CTP synthase (CTPS) is a key enzyme in de novo CTP synthesis, playing a critical role in nucleotide metabolism and cellular proliferation. Human CTPS1 (hCTPS1), one of the two CTPS isoforms, is essential for immune responses and is highly expressed in proliferating cells, making it a promising therapeutic target for immune-related diseases and cancer. hCTPS1 functions as a homotetramer, with each monomer comprising a glutamine amidotransferase (GAT) domain and an amidoligase (AL) domain. In the presence of GTP, the GAT domain hydrolyzes glutamine (Gln) to produce ammonia, which is transferred to the AL domain to catalyze the conversion of uridine triphosphate (UTP) to cytidine triphosphate (CTP) via an ATP-dependent intermediate, 4-phospho-UTP (4-Pi-UTP).

To stabilize the GAT domain, we included 6-diazo-5-oxo-L-norleucine (DON), a glutamine analog that irreversibly inhibits CTPS activity by covalently binding to the glutamine site. Using 312,573 particles for reconstruction, we achieved a final resolution of 3.3 Å. The structure showed that hCTPS1 filaments consist of helical arrays of tetramers, with each helical unit rising by 105 Å and twisting by approximately 40°. The tetramers are connected through α-helix-mediated interactions involving residues 346–357 in the GAT domain. Notably, residues H355 and W358, which are critical for filament assembly across species, exhibited continuous electron density in the density map, underscoring their conserved role. In our structure, two CTP molecules were observed bound to each protomer: one at the interface of three protomers (overlapping with the UTP binding site) and the other within a single protomer (overlapping with the ATP binding site). We designated these as the canonical and non-canonical binding pockets, respectively. In the canonical binding pocket, the triphosphate group of CTP is stabilized by electrostatic and hydrogen-bonding interactions with each protomer. In the non-canonical binding pocket, the triphosphate group interacts electrostatically with a loop, while the cytosine group is stabilized by interactions with S21, K319, and F77.

>MKYILVTGGVISGIGKGIIASSVGTILKSCGLHVTSIKIDPYINIDAGTFSPYEHGEVFVLDDGGEVDLDLGNYERFLDIRLTKDNNLTTGKIYQYVINKERKGDYLGKTVQVVPHITDAIQEWVMRQALIPVDEDGLEPQVCVIELGGTVGDIESMPFIEAFRQFQFKVKRENFCNIHVSLVPQPSSTGEQKTKPTQNSVRELRGLGLSPDLVVCRCSNPLDTSVKEKISMFCHVEPEQVICVHDVSSIYRVPLLLEEQGVVDYFLRRLDLPIERQPRKMLMKWKEMADRYDRLLETCSIALVGKYTKFSDSYASVIKALEHSALAINHKLEIKYIDSADLEPITSQEEPVRYHEAWQKLCSAHGVLVPGGFGVRGTEGKIQAIAWARNQKKPFLGVCLGMQLAVVEFSRNVLGWQDANSTEFDPTTSHPVVVDMPEHNPGQMGGTMRLGKRRTLFQTKNSVMRKLYGDADYLEERHRHRFEVNPVWKKCLEEQGLKFVGQDVEGERMEIVELEDHPFFVGVQYHPEFLSRPIKPSPPYFGLLLASVGRLSHYLQKGCRLSPRDTYSDRSGSSSPDSEITELKFPSINHD[4x]Proliferating Cell Nuclear Antigen (PCNA)—the eukaryotic sliding clamp—is an 86-kDa homotrimeric ring with a six-fold pseudosymmetric rotation axis running through the centre of the clamp and a central channel lined with lysine and arginine-rich α-helices through which DNA is threaded (1–6). The front face of the PCNA ring contains the site of interaction of polymerases and other proteins, named the PIP-box binding site. The PCNA–associated factor p15PAF (hereafter named p15) is an oncogenic, 11 kDa intrinsically disordered protein that regulates DNA replication and lesion bypass via a PIP-box interaction with PCNA. p15 co-localizes with PCNA in the nucleus of proliferating cells mainly in the S phase of the cell cycle. Thus, p15 outcompetes DNA for a common binding site in the clamp channel, and the stoichiometry of binding dictates the available sliding surfaces.

The co-crystal structure of PCNA in complex with two p15 molecules and a 10 bp primed DNA substrate, solved at 3.2 Å resolution, shows the duplex portion of DNA in the PCNA channel leaning towards the subunit not occupied by p15. Crystals including the p1550–77 peptide diffracted to 3.2 Å resolution, and the Fourier difference map calculated after placing and refining the PCNA ring alone in the asymmetric unit showed two PIP-box sites occupied by the p1550–77 peptide and electron density features in the channel that may be attributed to one strand of the DNA duplex. However, electron density from the second strand is weak and the 4-base single stranded overhang invisible. This suggests partial disorder and/or low occupancy of DNA. We then aligned the previously determined structure of PCNA bound to a 10 bp dsDNA onto the current model and found that the DNA duplex fits reasonably well the residual electron density in the ring channel. This DNA position, which leans towards the PCNA subunit not occupied by p1550–77, also results in the best model statistics, lowest B-factors of DNA and best quality of the 2Fo – Fc electron density map (and Supplementary Table ST2) and, importantly, agrees with the results from MD simulations (see below). As in the p1550–77–PCNA binary structure, the stoichiometry of p1550–77 binding to PCNA is defined by the crystal packing, where a symmetry-related PCNA molecule occludes the peptide binding site on one subunit. The peptide with higher occupancy has its PIP-box (Q62-F69) sitting on at the PCNA front face forming a 310 helical turn, with a type-I β-turn at its N-terminus (P59-Q62) that positions residues P52-T58 to contact PCNA helices αA2 and αB2 on the clamp inner wall. The p15 residues N-terminal to the PIP-box contact four helices on the ring inner wall, partly shielding the DNA binding site of two subunits.

>[2x]MFEARLVQGSILKKVLEALKDLINEACWDISSSGVNLQSMDSSHVSLVQLTLRSEGFDTYRCDRNLAMGVNLTSMSKILKCAGNEDIITLRAEDNADTLALVFEAPNQEKVSDYEMKLMDLDVEQLGIPEQEYSCVVKMPSGEFARICRDLSHIGDAVVISCAKDGVKFSASGELGNGNIKLSQTSNVDKEEEAVTIEMNEPVQLTFALRYLNFFTKATPLSSTVTLSMSADVPLVVEYKIADMGHLKYYLAPK;> HMFEARLVQGSILKKVLEALKDLINEACWDISSSGVNLQSMDSSHVSLVQLTLRSEGFDTYRCDRNLAMGVNLTSMSKILKCAGNEDIITLRAEDNADTLALVFEAPNQEKVSDYEMKLMDLDVEQLGIPEQEYSCVVKMPSGEFARICRDLSHIGDAVVISCAKDGVKFSASGELGNGNIKLSQTSNVDKEEEAVTIEMNEPVQLTFALRYLNFFTKATPLSSTVTLSMSADVPLVVEYKIADMGHLKYYLAPKI;>PVCVRPTPKWQKGIGEFFRL[2x]>MPVFTASFQCVTLFGQPASAADAQPLLQGQRPFLHLHARRRRPCGPMLISKSPPYPASEETREWEADGQHEHTDELRETTTTMIDGIRTALRSIGEGEISISAYDTSLVALLKRLDGGDGPQFPSTIDWIVQNQLPDGSWGDASFFMMGDRIMSTLACVVALKSWNIHTDKCERGLLFIQENMWRLAHEEEDWMLVGFEIALPSLLDMAKDLDLDIPYDEPALKAIYAERERKLAKIPRDVLHSMPTTLLHSLEGMVDLDWEKLLKLRCLDGSFHCSPASTATAFQQTGDQKCFEYLDGIVKKFNGGVPCIYPLDVYERLWAVDRLTRLGISRHFTSEIEDCLDYIFRNWTPDGLAHTKNCPVKDIDDTAMGFRLLRLYGYQVDPCVLKKFEKDGKFFCLHGESNPSSVTPMYNTYRASQLKFPGDDGVLGRAEVFCRSFLQDRRGSNRMKDKWAIAKDIPGEVEYAMDYPWKASLPRIETRLYLDQYGGSGDVWIGKVLHRMTLFCNDLYLKAAKADFSNFQKECRVELNGLRRWYLRSNLEKFGGTDPQTTLMTSYFLASANIFEANRAAERLGWARVALLADAVSSHFRRIGGPKNSTSNLEELISLVPFDDAYSGSLREAWKQWLMAWTAKESSQESIEGDTAILLVRAIEIFGGRHVLTGQRPDLWEYSQLEQLTSSICCKLSRRVLAQENGESTEKVEEIDQQVDLEMQELTRRVLQGCSAINRLTRETFLHVVKSFCYVAYCSPETIDSHIDKVIFQDVIEFHHHHHH[6x]

The large superfamily of labdane-related diterpenoids is defined by the cyclization of linear geranylgeranyl pyrophosphate (GGPP), catalyzed by copalyl diphosphate synthases (CPSs) to form the basic decalin core, the copalyl diphosphates (CPPs). Here, we used X-ray crystallography and cryo-EM methods to describe different oligomeric structures of a syn-copalyl diphosphate synthase from Oryza sativa (OsCyc1), and provided a cryo-EM structure of OsCyc1D367A mutant in complex with the substrate GGPP. The structure of monomer OsCyc1 consists of an αβγ domain and a catalytic center located between the β and γ domains. OsCyc1 catalyzes GGPP to form syn-CPP, in which new bonds form between C6 and C11, as well as between C10 and C15.

To determine the structure of OsCyc1, we used the stable N-terminal truncation variant of OsCyc1, OsCyc169–767, from which the plastid targeting peptide was removed. Next, we determined the crystal structure of OsCyc169–767 by molecular replacement method at 3.5 Å resolution, which contains six protomers (Chains A/B/C/D/E/F) in the asymmetric unit. The overall structure of monomer OsCyc1 is similar to that of AtCPS, AgAS and SmMDS, with RMSD values for Cα of 1.86 Å, 2.15 Å and 1.94 Å, respectively. As the crystal structure of OsCyc1 was solved at a higher resolution than its cryo-EM structures, particularly in the γ domain region, we focused on utilizing the crystal structure to analyze oligomer interactions. Residues located within or near α22 interact with residues in α25, such as Q627 with R720, which are at a hydrogen bonding distance in the crystal structure. The interactions between α23 and α24 include R652 with Q675, as well as E640 with K686, possibly through van der Waals interactions. In addition, we found that H-bonds form between S674 and E677 within the α24 helix. When we analyzed the binding interactions in the crystal structure, we found that the interactions between different dimers are similar. The interaction between dimer C/D and dimer E/F is identical to the interaction between dimer A/B and dimer C/D, suggesting that a pseudo-twofold symmetry axis exists between the chains C and D. In addition to the abovementioned interactions in the center of the hexamer, a linkage exists in the γ domain of protomer B and protomer E, which protrude to the edge of the crystal hexamer structure. In the crystal structure of OsCyc1, the distance between the d1-oxygen in D367 and the d2-nitrogen in the conserved N414 is 2.97 Å.>[2x]GIENIPATLSHGGRFIQYNIFGNIFEVTAKYKPPIMPIGKGAYGIVCSAMNSETNESVAIKKIANAFDNKIDAKRTLREIKLLRHMDHENIVAIRDIIPPPLRNAFNDVYIAYELMDTDLHQIIRSNQALSEEHCQYFLYQILRGLKYIHSANVLHRDLKPSNLLLNANCDLKI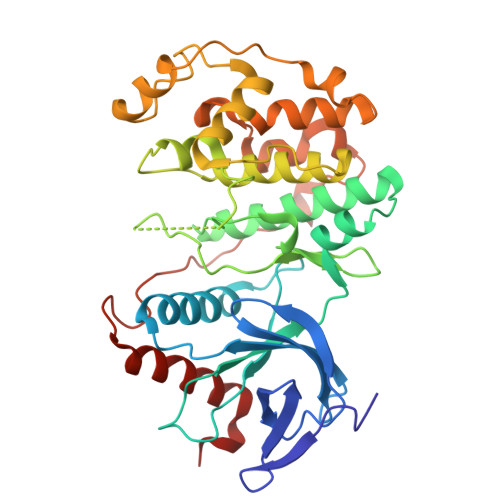CDFGLARVTSESDFMTEYVVTRWYRAPELLLNSSDYTAAIDVWSVGCIFMELMDRKPLFPGRDHVHQLRLLMELIGTPSEEELEFLNENAKRYIRQLPPYPRQSITDKFPTVHPLAIDLIEKMLTFDPRRRITVLDALAHPYLNSLHDISDEPECTIPFNFDFENHALSEEQMKELIYREALAFNPEYQQ>MKLSARNQLAGKVVSIKEGAVNGIVVLDIGGGNQISSTISMDSIRELGLQVGSDAYAVIKATSVMIGIDDW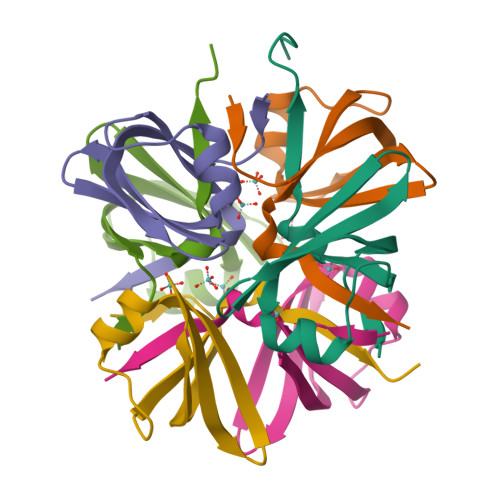SHP[6x]>MGSSHHHHHHSSGLVPRGSHTGAGLRWKHTSSLKVANEPVLAFTQGSPERDALQKALKDLKGRMEAIPCVVGDEEVWTSDVQYQVSPFNHGH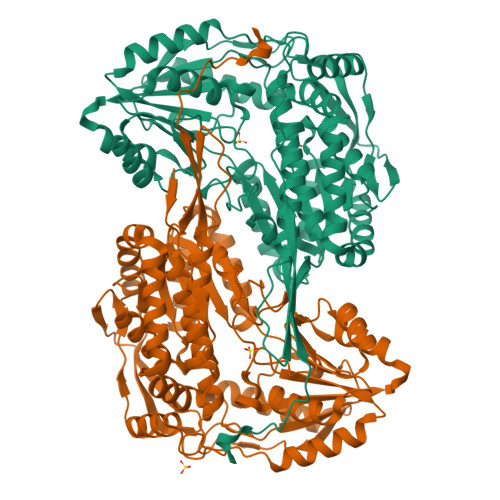KVAKFCYADKSLLNKAIEAALAARKEWDLKPIADRAQIFLKAADMLSGPRRAEILAKTMVGQGKTVIQAEIDAAAELIDFFRFNAKYAVELEGQQPISVPPSTNSTVYRGLEGFVAAISPFNFTAIGGNLAGAPALMGNVVLWKPSDTAMLASYAVYRILREAGLPPNIIQFVPADGPLFGDTVTSSEHLCGINFTGSVPTFKHLWKQVAQNLDRFHTFPRLAGECGGKNFHFVHRSADVESVVSGTLRSAFEYGGQKCSACARLYVPHSLWPQIKGRLLEEHSRIKVGDPAEDFGTFFSAVIDAKSFARIKKWLEHARSSPSLTILAGGKCDDSVGYFVEPCIVESKDPQEPIMKEEIFGPVLSVYVYPDDKYKETLQLVDSTTSYGLTGAVFSQDKDVVQEATKVLRNAAGNFYINDKSTGSIVGQQPFGGARASGTNDKPGGPHYILRWTSPQVIKETHKPLGDWSYAYMQ[4x]>[2x]SDHSIEVTFRVKTQQVIIPEQNIRGNELPLRRWQMELLMLDATGKEVEPTILSKCIYHLHSSFKQPKRRLNSLPFFIKET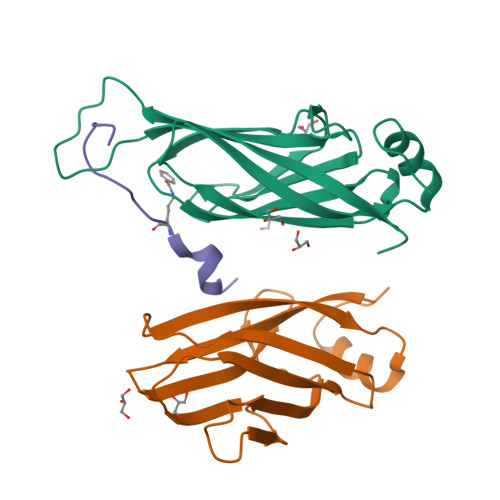GWGEFNLKIECFFIGNAGKFSIEHDLTFEDDAYAVDYTVDVPHEFSHLNSELSKYFDLP;> KQLASKAARKSAPSTGGVKY>TQSLHHSSSREALTDIIMDAKIRKNLTFEAINEGTGLSLAFV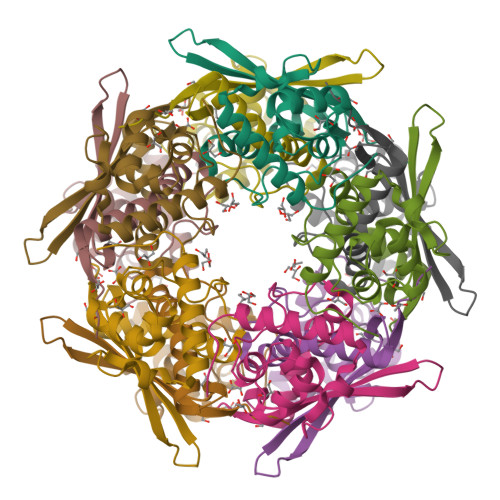TAALLGQHPLPEQAARVVAAKLDLDEDAVRLLQTIPLRGSIPSGVPTDPTIYRFYEMVQIYGSTLKALVHEQFGDGIISAINFKLDIKKVPDPDGGERAVITLDGKYLPTKPF[10x]> EELQVDCNTLSSMPNVSFTIGGKKFGLTPEQYILKVGKGEATQCISGFTAMDATLLGPLWILGDVFMRPYHT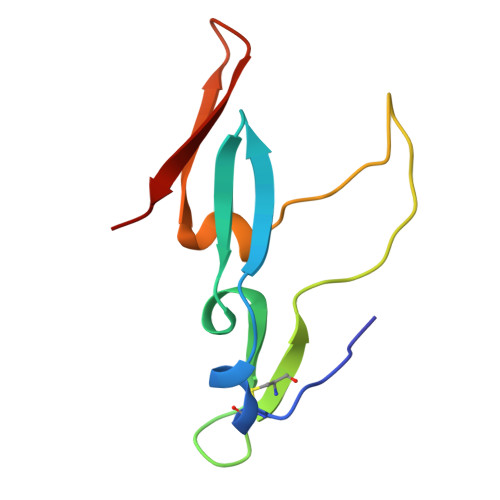VFDYGNLLVGFAEAA(2R,3R)-2-(carboxymethoxy)-4-{[5-(naphthalen-2-yl)pentyl]amino}-3-{[5-(naphthalen-2-yl)pentyl]oxy}-4-oxobutanoic acid | 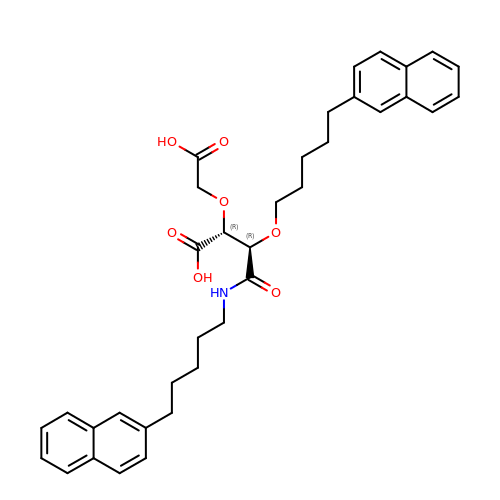C36 H41 N O7 | MMKNOJATXTZICP-KKLWWLSJSA-N>[4x]SNAMTDSTTELTPAAPVSWPDGKTCAVAFTFDVDAESPLLTTDPAFADRMGTMS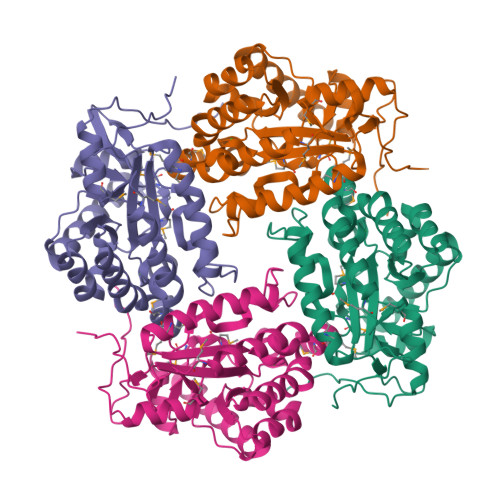HQAYGPLVGVPRLLGILDEFNVPGTFFVPGYTAHRHPEPIRSIARAGHEIAHHGYLHESLVGADEDTERKILTRGIEALEEVAGVHPVGYRAPMWEMNWHTPKLLAEFGFLYDSTLMDSDHPYELAVGDGSLVELPVSWALDDWQQYCFVPDFSGTGLIETPAKAIELWRAELNAMRDIGGAWVLTNHPFLSGRPGRAAALREFIAEVCAMDDVWVAGMSQIAEHVRAQKLTPRTLTRPELTPVAE>[3x]MPRPRVLLLGDPARHLDDLWSDFQQKFEVIPANLTTHDGFKQALREKRYGDFEAIIKLAVENGTESYPWNADLISHLPSSLKVFAAAGAGFDWLDLDALNERGVAFANSRGAGDTATSDLALYLILSVFRLASYSERAARTGDPETFNRVHLEIGKSAHNPRGHVLGAVGLGAIQKEIARKAVHGLGMKLVYYDVAPADAETEKALGAERVDSLEELARRSDCVSVSVPYMKLTHHLIDEAFFAAMKPGSRIVNTARGPVISQDALIAALKSGKLLSAGLDVHEFEPQVSKELIEMKHVTLTTHIGGVAIETFHEFERLTMTNIDRFLLQGKPLLTPAGKVFAPSSAA;> MPRPRVLLLGDPARHLDDLWSDFQQKFEVIPANLTTHDGFKQALREKRY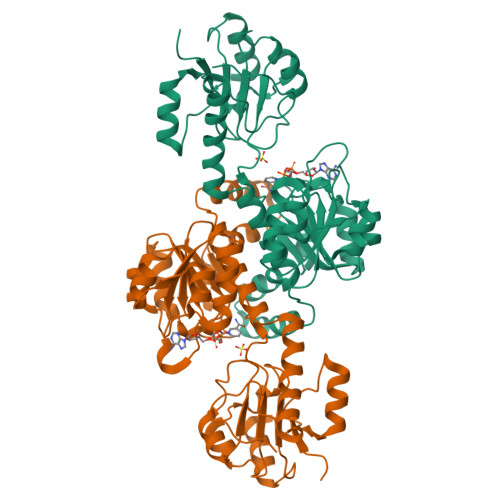GDFEAIIKLAVENGTESYPWNADIISHLPSSLKVFAAAGAGFDWLDLDALNERGVAFANSRGAGDTATSDLALYLILSVFRLASYSERAARTGDPETFNRVHLEIGKSAHNPRGHVLGAVGLGAIQKEIARKAVHGLGMKLVYYDVAPADAETEKALGAERVDSLEELARRSDCVSVSVPYMKLTHHLIDEAFFAAMKPGSRIVNTARGPVISQDALIAALKSGKLLSAGLDVHEFEPQVSKELIEMKHVTLTTHIGGVAIETFHEFERLTMTNIDRFLLQGKPLLTPAGKVFAPSSAA> ADVPAGVQLADKQTLVRNNGSEVQSLDPHKIEGVPESNVSRDLFEGLLISDVEGHPSPGVAEKWENKDFKVWTFHLRENAKWSDGTPVTAHDFVYSWQRLADPNTASPYASYLQYGHIANIDDIIAGKKPATDLGVKALDDHTFEVTLSEPVPYFYKLLVHPSVSPVPKSAVEKFGDKWTQPANIVTNGAYKLKNWVVNERIVLERNPQYWDNAKTVINQVTYLPISSEVTDVNRYRSGEIDMTYNNMPIELFQKLKKEIPNEVRVDPYLCTYYYEINNQKAPFNDVRVRTALKLALDRDIIVNKVKNQGDLPAYSYTPPYTDGAKLVE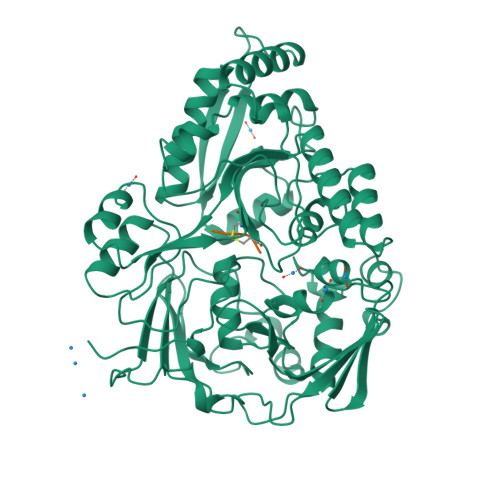PEWFKWSQQKRNEEAKKLLAEAGFTADKPLTFDLLYNTSDLHKKLAIAVASIWKKNLGVNVNLENQEWKTFLDTRHQGTFDVARAGWCADYNEPTSFLNTMLSDSSNNTAHYKSPAFDKLIADTLKVADDTQRSELYAKAEQQLDKDSAIVPVYYYVNARLVKPWVGGYTGKDPLDNIYVKNLYIIKH;> KKKA> GGMQHNLIAFLSDVGSADEAHALCKGVMYGVAPAATIVDITHDVAPFDVREG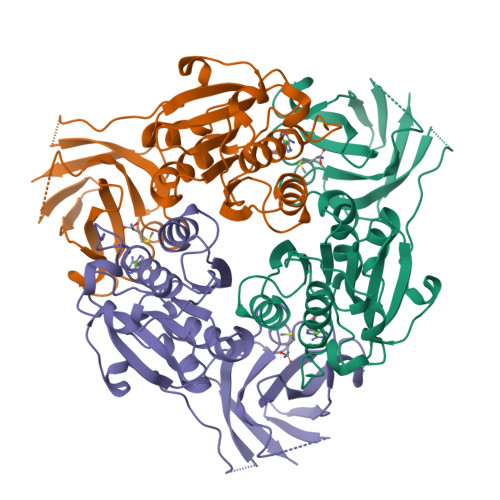ALFLADVPHSFPAHTVICATVYPETGTATHTIAVRNEKGQLLVGPNNGLLSFALDASPAVECHEVLSPDVMNQPVTPTWYSKDIVAACAAHLAAGTDLAAVGPRIDPKQIVRLPYASASEVEGGIRGEVVRIDRAFGNVWTNIPTHLIGSMLQDGERLEVKIEALSDTVLELPFCKTFGEVDEGQPLLYLNSRGRLALGLNQSNFIEKWPVVPGDSITVSPRVPDSNLGPVLG> MEELFNALPQPLQQLSLALAGEIPLTDHIFEQAASTWHVQPRSLTYKLLDHIPFATPVVVPPSIYHSLDWSKCFAVNQDRVERIPTIDNPDDVYVPNSDIGPLLTSLHTIPDYGFLHPTIENDATTLRAERARCASTFYKIASSQARQVKLDPIRMLGFLLLVQARPRVPSGLVTDQPTRRDPTLSPALHAIWQVMQYYKVAGVYYAPALVVPSGAIWWIPPPGKRNVVSVQYLLTDLISLAILAHMTDMSPTLELTGVLMYLRAASSHSYAYTLLQMKSVFPALSLRSMYRNKGFGGKAPAIEWTEPRSKYKFRWTGVTQLHDGLRPRSPSMDVPTLETLAKYELVDIGHTIIRERNAHPQHNHDSVRFVRDVMALTSGMYLVRQPTMSVLREYSQVPDIKDPIPPSAWTGPIGNVRYLLPSVQGPARHLYDTWRAAARQIAQDPQWHDPLNQAIMRAQYVTARGGSSASLKFALKVTGIVLPEYDDSKVKKSSKIYQAAQIARIAFMLLIAAIHAEVTMGIRNQVQRRARSIMPLNVIQQAISAPHTLVANYINKHMNLSTTSGSVVTDKVIPLILYASTPPNTVVNVDIKACDASITYNYFLSVICGAMHEGFEVGNADAAFMGVPSTIVSDRRSPVAPYSRPISGLQTMVQHLADLYAAGFRYSVSDAFSSGNKFSFPTSTFPSGSTATSTEHTANNSTMMEYFLNVHAPSHVKSASLKRILTDMTIQRNYVCQGDDGILLLPHEAASKISADDMNELLTCLRDYGQLFGWNYDIDWSDTAEYLKLYALMGCRIPNTSRHPPVGKEYAAPQTDEIWPSLIDIVIGHHLNGVTDVLNWREWLRFSWAFACYSSRGGYTNPRGQSFSAQYPWWTFVYLGIPPILLPGQTPFIHSCYMPPGDQGMFSILNGWRDWLISHASTTLPPLRHNHPVWGLSDVPSLLSQFGVYAGYHAAQHYRRPKPAPETASSDSINQITSDLTEYLFYDSALKARVMKGRYNWERLSSSLSLNVGSRVPSLFDVPGKWVAAGRDAEKPPPSSVEDMFTSLNRCIRRPTHSFSRLLELYLRVHVALGESIPLAIDPDVPQVAGADPANDDH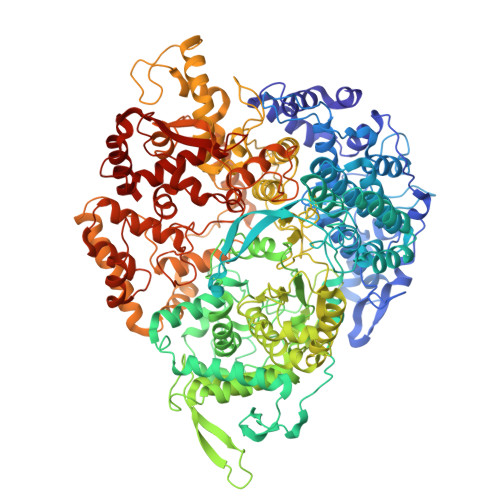WFKYTCLGDIPSATRNYFGESLFVGRVVSGLDVEAVDATLLRLKILGAPPEAFIAVLNGIGMSDSEAHQIAGRISLANAQLVQIARVVHLSIPSSWMTLNTGPYIHHHAYDFKPGITQPSAKSRDKSIWMSPILKLLCTSYAMTVAGPVRTSIVTEIDGSAAALSGNLRVWMRDV>[2x]SNAMSAFITFEGPEG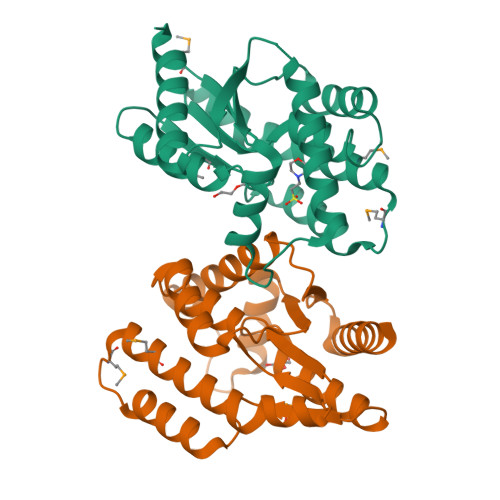SGKTTVINEVYHRLVKDYDVIMTREPGGVPTGEEIRKIVLEGNDMDIRTEAMLFAASRREHLVLKVIPALKEGKVVLCDRYIDSSLAYQGYARGIGVEEVRALNEFAINGLYPDLTIYLNVSAEVGRERIIKNSRDQNRLDQEDLKFHEKVIEGYQEIIHNESQRFKSVNADQPLENVVEDTYQTIIKYLEKI>MKNNKIYLLGACLLCAVTTFAQNVSLQPPPQQLIVQNKTIDLPAVYQLNGGEEANPHAVKVLKELLSGKQSSKKGMLISIGEKGDKSVRKYSRQIPDHKEGYYLSVNEKEIVLAGNDERGTYYALQTFAQLLKDGKLPEVEIKDYPSVRYRGVVEGFYGTPWSHQARLSQLKFYGKNKMNTYIYGPKDDPYHSAPNWRLPYPDKEAAQLQELVAVANENEVDFVWAIHPGQDIKWNKEDRDLLLAKFEKMYQLGVRSFAVFFDDISGEGTNPQKQAELLNYIDEKFAQVKPDINQLVMCPTEYNKSWSNPNGNYLTTLGDKLN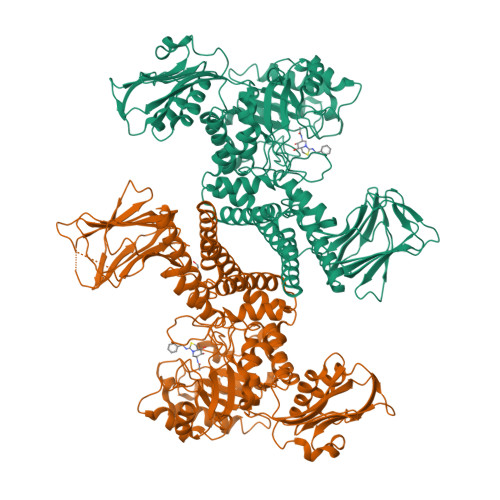PSIQIMWTGDRVISDITRDGISWINERIKRPAYIWWNFPVSDYVRDHLLLGPVYGNDTTIAKEMSGFVTNPMEHAESSKIAIYSVASYAWNPAKYDTWQTWKDAIRTILPSAAEELECFAMHNSDLGPNGHGYRREESMDIQPAAERFLKAFKEGKNYDKADFETLQYTFERMKESADILLMNTENKPLIVEITPWVHQFKLTAEMGEEVLKMVEGRNESYFLRKYNHVKALQQQMFYIDQTSNQNPYQPGVKTATRVIKPLIDRTFATVVKFFNQKFNAHLDATTDYMPHKMISNVEQIKNLPLQVKANRVLISPANEVVKWAAGNSVEIELDAIYPGENIQINFGKDAPCTWGRLEISTDGKEWKTVDLKQKESRLSAGLQKAPVKFVRFTNVSDEEQQVYLRQFVLTIEKK[2x]2-[1-({2-[2-(dimethylamino)-1H-benzimidazol-1-yl]-9-methyl-6-(morpholin-4-yl)-9H-purin-8-yl}methyl)piperidin-4-yl]propan-2-ol 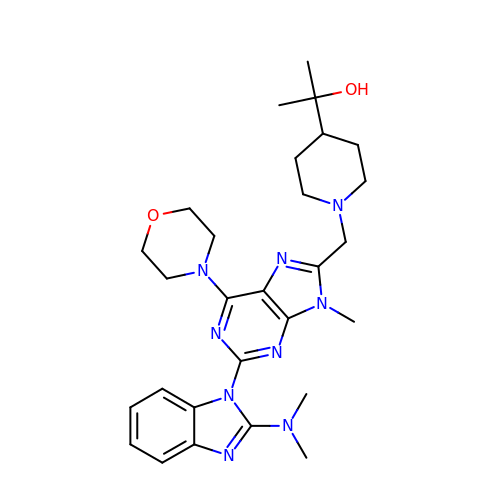| C28 H39 N9 O2 | SUPBDTZKRDSWGT-UHFFFAOYSA-N Sirtuins generally catalyze the deacylation of modified lysine residues in protein substrates coupled with the breakdown of NAD+ into nicotinamide (NAM) and 2'-O-acyl-ADP-ribose. To address this, we developed an engineered hSIRT1 (mini-hSIRT1) that is biochemically equivalent to the full-length enzyme with respect to basal catalytic activity and activation by STACs. Mini-hSIRT1 comprises a catalytic domain that assumes a Rossmann-fold large lobe and a zinc-binding small lobe common to all sirtuins, an N-terminal three-helical bundle encompassing the SBD and a C-terminal β-hairpin CTR peptide18.

X-ray crystallographic analysis of mini-hSIRT1 resulted in the first detailed structural determination of a fully functional human SIRT1 with a bound small molecule activator. The N-terminal SBD forms an independently folded, three-helix bundle with 1 binding to the helix-turn-helix (H2-T-H3) motif within the SBD, consistent with the HDX-MS and enzyme kinetic results. STAC 1 interacts extensively with the hydrophobic side chains of Leu206, Thr209 (methyl), Pro211, Pro212, Leu215, Thr219 (methyl), Ile223 and Ile227 from the H2-T-H3 motif with only one hydrophilic interaction: a hydrogen bond with Asn226. The major mini-hSIRT1/1-binding site is a shallow hydrophobic surface depression with an off-center, deeper hydrophobic pocket, that the CF3 group of 1 occupies. This is consistent with the observed structure-activity relationships developed across multiple STAC chemotypes, indicating the requirement of overall flatness of the core scaffold maintained by an intramolecular hydrogen bond. In the crystal structure, Ile223 lies directly beneath the STAC and lines the pocket into which the meta-CF3 of 1 inserts. Asn226 appears to form a hydrogen bond between its carboxamide nitrogen and the carbonyl oxygen of 1 on the surface of the protein. Interestingly, a STAC-mediated dimer of mini-hSIRT1 related by crystallographic symmetry was observed in the crystal lattices. Comparison of the three structures shows that the locations of the N-terminal SBD domain relative to the catalytic core are divergent among the three structures, likely to be impacted by different crystal packings.

> GPYTFVQQHLMIGTDPRTILKDLLPETIPPPELDDMTLWQIVINILSEPPKRKKRKDINTIEDAVKLLQECKKIIVLTGAGVSVSCGIPDFRSRDGIYARLAVDFPDLPDPQAMFDIEYFRKDPRPFFKFAKEIYPGQFQPSLCHKFIALSDKEGKLLRNYTQNIDTLEQVAGIQRIIQCHGSFATASCLICKYKVDCEAVRGDIFNQVVPRCPRCPADEPLAIMKPEIVFFGENLPEQFHRAMKYDKDEVDLLIVIGSSLKVRPVALIPSSIPHEVPQILINREPLPHLHFDVELLGDCDVIINELCHRLGGEYAKLCCNPVGGGSGGGSQYLFLPPNRYIFHGAEVYSDSEDDV>[2x]MDLPKAYDPKSVEPKWAEKWAKNPFVANPKSGKPPFVIFMPPPNVTGSLHMGHALDNSLQDALIRYKRMRGFEAVWLPGTDHAGIATQVVVERLLLKEGKTRHDLGREKFLERVWQWKEESGGTILKQLKRLGASADWSREAFTMDEKRSRAVRYAFSRYYHEGLAYRAPRLVNWCPRCETTLSDLEVETEPTPGKLYTLRYEVEGGGFIEIATVRPETVFADQAIAVHPEDERYRHLLGKRARIPLTEVWIPILADPAVEKDFGTGALKVTPAHDPLDYEIGERHGLKPVSVINLEGRMEGERVPEALRGLDRFEARRKAVELFREAGHLVKEEDYTIAL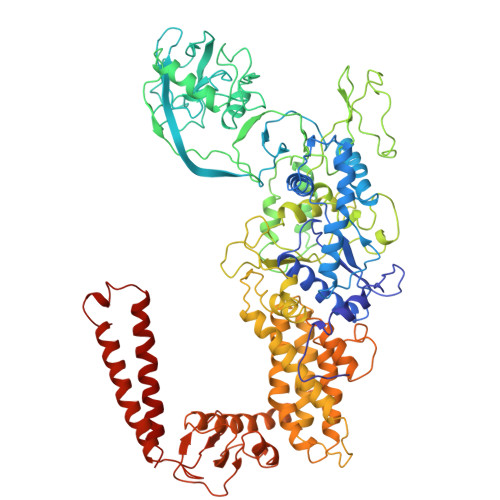ATCSRCGTPIEYAIFPQWWLRMRPLAEEVLKGLRRGDIAFVPERWKKVNMDWLENVKDWNISRQLWWGHQIPAWYCEDCQAVNVPRPERYLEDPTSCEACGSPRLKRDEDVFDTWFSSALWPLSTLGWPEETEDLKAFYPGDVLVTGYDILFLWVSRMEVSGYHFMGERPFKTVLLHGLVLDEKGQKMSKSKGNVIDPLEMVERYGADALRFALIYLATGGQDIRLDLRWLEMARNFANKLYNAARFVLLSREGFQAKEDTPTLADRFMRSRLSRGVEEITALYEALDLAQAAREVYELVWSEFCDWYLEAAKPALKAGNAHTLRTLEEVLAVLLKLLHPMMPFLTSELYQALTGKEELALEAWPEPGGRDEEAERAFEALKQAVTAVRALKAEAGLPPAQEVRVYLEGETAPVEENLEVFRFLSRADLLPERPAKALVKAMPRVTARMPLEGLLDVEEWRRRQEKRLKELLALAERSQRKLASPGFREKAPKEVVEAEEARLKENLEQAERIREALSQIG>[2x]GPMETTNWIGDENLTGNAEAPAKDDVVPDKNQFRYQKEELAAFCHFGPNTFNEIEWGEHYGNQKPSEIFTLKNDFDAETLVKTLKDAGFKKLIVTAKHHDGFCIWDSEHTEYDVKASGYKNKNGESDILAEISKACTDQNMDMGLYLSPWDIHEPSYGYKDEHGNPTTPDKDAKDYNEFYNNQLEEILGNPKYGNDGHFVEVWMAGAKGSGANAQEYDFKKWFKTIQDNEGKAAGYDADCMLFGAEAYTTVRWIGNELGIAGKDTWSKSKVDKDKNTINSNKQGNATVGFEDGDQWTVPEADARITSGWFWGTKKNTPKTMEELSDMYFNSVGHNATLLLNVPPNNQGTVDKAILDRVTEFGNNIKATFKTNLAKAEGASVKVSEVRGGAKEYKPGNMIDDNDETYWATSDGKKSGEILIDLGKETKFDVVSIEEAIQNGQRINNYKVEYRNGDSGTWTLLEEGKTIGAKRLCRTSETTARQIKITVGTCDGKVPMISEIGVYKSTEDMEKPNPIPKGMEVIDVEDKDVADGKGFTFKGKWNPENQPQYING

To access this source of nutrients, gut bacteria encode α-l-fucosidases (fucosidases) which catalyze the hydrolysis of terminal α-l-fucosidic linkages. We identified and characterized a fucosidase from R. gnavus E1 with the capacity to recognize fucosylated glycans capped with sialic acid and to hydrolyze α1–3/4 fucosyl linkages in these substrates without the need to remove sialic acid. The enzymatic characterization of R. gnavus fucosidases focused on previously uncharacterized bacterial fucosidases revealed that fucosidase ATCC_03833 belongs to GH29-A while E1_10125 belongs to GH29-B subfamily. The enzyme consists of two distinct domains, a catalytic domain (PF001120) domain comprising residues 46–366 in N-terminal and a F5/8 Type C domain (PF00754) covering residues 385–526 in C-terminal.

In an attempt to obtain crystal structures in complex with the substrate, an active site mutant (E1_10125 D221A) was generated. However, following co-crystallization experiments with 2′FL, fucose was found bound in the active site, indicating residual fucosidase activity. Clear electron density was present for both α- and β-fucose anomers. It was not possible to obtain crystals of E1_10125 D221A in the absence of 2′FL. Attempts were made to displace the fucose molecule with other fucosylated ligands; however, these were unsuccessful, perhaps due to the substrate binding site being present at a tightly packed interface between two symmetry related protein molecules. Following 500 ns MD simulations of the E1_10125 D221A mutant and docking of the sLeX ligand, the molecular model showed that sialic acid ring sits in the neighboring subsite. Polar contacts are established between nearby residues, Glu262 and Trp269; in particular, and hydroxyl groups present at sialic acid C4, C8 and C9 positions. This analysis confirmed that the E1_10125 fucosidase enzyme shows an open binding site able to accommodate the sLeX ligand.>[4x]MAHHHHHHVDDDDKENLYFQSKPNLSAKDLALLLFTHLPGNNTPFHILAQVLSKIAYKSGKSGAFLDAFHQILSEGENAQAALTRLSRTFDAFLGVVPPVIRVKNFQTVPRPCQKSLRAVPPNPTIDKGWVCVYSSEQGETRALKI

Filoviruses encode a viral protein termed VP35 which is important for nucleocapsid assembly, replication and transcription and also plays a critical role in host immunosuppression. VP35 binds to and likely masks viral dsRNA from host factors, which leads to suppression of RNA silencing, inhibition of phosphorylation/activation of interferon regulatory factor 3 (IRF-3) and antagonism of the type I IFN response. Here we present the crystal structure of the dsRNA-binding domain (RBD) of Marburg virus VP35, alone and in complex with dsRNA. The structures and accompanying dsRNA-binding analysis performed by dot-blot assays and isothermal titration calorimetry reveal that MARV VP35 RBD coats the sugar-phosphate backbone along the length of dsRNA in addition to capping at the terminus, suggesting an alternate mechanism of dsRNA masking for immunosuppression.

MARV VP35 RBD was crystallized in complex with a 12-bp dsRNA oligonucleotide. Data were complete to 2.5 Å resolution and the structure was determined by molecular replacement in space group P21. The asymmetric unit contains four molecules of the VP35 RBD bound to one molecule of 12-bp dsRNA. Interpretable electron density was observed for residues 208–329 of the RBD and all 24 bases of the dsRNA. The MARV VP35 RBD protomers from the complex align with the unliganded MARV VP35 RBD with an r.m.s.d. of 0.44 Å suggesting no appreciable secondary structural changes occur upon dsRNA binding. By contrast, in the MARV VP35 complex structure, the terminal bases of each dsRNA in the asymmetric unit stack with those of the dsRNA in a neighboring asymmetric unit. Thus, in these crystals, the dsRNA molecules together assemble one, pseudo-continuous dsRNA helix. The four MARV VP35 RBDs in the asymmetric unit do not end-cap, but instead, solely bind along the sugar-phosphate backbone, forming a continuous spiral of VP35 RBDs along the dsRNA. This arrangement results in a complete coating of the dsRNA by VP35 RBDs, with each of the conserved, central basic patches of VP35 RBD facing the dsRNA sugar-phosphate backbone. Each VP35 RBD–dsRNA interaction involves ∼520 Å2 of buried surface and is accomplished by direct hydrogen bonds between N261, Q263, T267, R271, S299, and I329 and the ribose-phosphate dsRNA backbone.> MDKELDGRFERLEKALATMIDSLSKNNPSTKLAQDLVAAEAELLEGLKLLEAHQNNHARIQQLRQSTEQADAQIKDIISSLWKM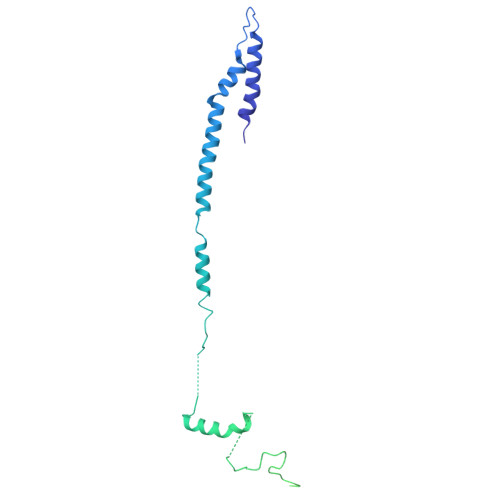RQELTSVQTSPIPKGAKFQFTTGELLDFARRISRNTLPPPGVTNGVNMTPAAARHSQQPSSVEPEDSFRVTSQSQTQTPNTSFNVSFNGTLVDTPGPFNNNSTPIPNAGPANSQNPHTELPEHLKLATNPLHGASFFPWPSVEQVRSGALGAYQLLVDKGIDPRGYDPEFEEQRRKDAEREAEERAKQEREEAERRAREEAERIARQRELERQRARESMAAAAEEGRRDSVVGGPAAGKPKQFTFLGGDDDDDDDDD> DYKDDDDKMPLAFCGTENHSAAYRVDQGVLNNGCFVDALNVVPHVFLLFITFPILFIGWGSQSSKVHIHHSTWLHFPGHNLRWILTFILLFVLVCEIAEGILSDGVTESRHLHLYMPAGMAFMAAITSVVYYHNIETSNFPKLLIALLIYWTLAFITKTIKFVKFYDHAIGFSQLRFCLTGLLVILYGMLLLVEVNVIRVRRYIFFKTPREVKPPEDLQDLGVRFLQPFVNLLSKGTYWWMNAFIKTAHKKPIDLRAIAKLPIAMRALTNYQRLCVAFDAQARKDTQSPQGARAIWRALCHAFGRRLILSSTFRILADLLGFAGPLCIFGIVDHLGKENHVFQPKTQFLGVYFVSSQEFLGNAYVLAVLLFLALLLQRTFLQASYYVAIETGINLRGAIQTKIYNKIMHMSTSNLSMGEMTAGQICNLVAIDTNQLMWFFFLCPNLWTMPVQIIVGVILLYYILGVSALIGAAVIILLAPVQYFVATKLSQAQRTTLEHSNERLKQTNEMLRGMKLLKLYAWESIFCSRVEVTRRKEMTSLRAFAVYTSISIF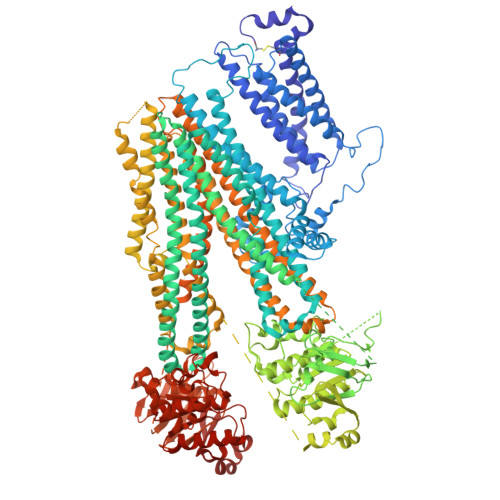MNTAIPIAAVLITFVGHVSFFKESDLSPSVAFASLSLFHILVTPLFLLSSVVRSTVKALVSVQKLSEFLSSAEIREEQCAPREPAPQGQAGKYQAVPLKVVNRKRPAREEVRDLLGPLQRLAPSMDGDADNFCVQIIGGFFTWTPDGIPTLSNITIRIPRGQLTMIVGQVGCGKSSLLLATLGEMQKVSGAVFWNSNLPDSEGEDPSSPERETAAGSDIRSRGPVAYASQKPWLLNATVEENITFESPFNKQRYKMVIEACSLQPDIDILPHGDQTQIGERGINLSGGQRQRISVARALYQQTNVVFLDDPFSALDVHLSDHLMQAGILELLRDDKRTVVLVTHKLQYLPHADWIIAMKDGTIQREGTLKDFQRSECQLFEHWKTLMNRQDQELEKETVMERKASEPSQGLPRAMSSRDGLLLDEEEEEEEAAESEEDDNLSSVLHQRAKIPWRACTKYLSSAGILLLSLLVFSQLLKHMVLVAIDYWLAKWTDSALVLSPAARNCSLSQECDLDQSVYAMVFTLLCSLGIVLCLVTSVTVEWTGLKVAKRLHRSLLNRIILAPMRFFETTPLGSILNRFSSDCNTIDQHIPSTLECLSRSTLLCVSALTVISYVTPVFLVALLPLAVVCYFIQKYFRVASRDLQQLDDTTQLPLVSHFAETVEGLTTIRAFRYEARFQQKLLEYTDSNNIASLFLTAANRWLEVCMEYIGACVVLIAAATSISNSLHRELSAGLVGLGLTYALMVSNYLNWMVRNLADMEIQLGAVKRIHALLKTEAESYEGLLAPSLIPKNWPDQGKIQIQNLSVRYDSSLKPVLKHVNTLISPGQKIGICGRTGSGKSSFSLAFFRMVDMFEGRIIIDGIDIAKLPLHTLRSRLSIILQDPVLFSGTIRFNLDPEKKCSDSTLWEALEIAQLKLVVKALPGGLDAIITEGGENFSQGQRQLFCLARAFVRKTSIFIMDEATASIDMATENILQKVVMTAFADRTVVTIAHRVHTILSADLVMVLKRGAILEFDKPETLLSQKDSVFASFVRADK>YLSIAFPENTKLDWKPVTKNTRYCPMGGEWFLEPGLQEESFLSSTPIGATPSKSDGFLCHAAKWVTTCDFRWYGPKYITHSIHNIKPTRSDCDTALASYKSGTLVSLGFPPESCGYASVTDSEFLVIMITPHHVGVDDYRGHWVDPLFVGGECDQSYCDTIHNSSVWIPADQTKKNICGQSFTPLTVTVAYDKTKEIAAGGIVFKSKYHSHMEGARTCRLSYCGRNGIKFPNGEWVSLDVKTRIQEKHLLPLFKECPAGTEVRSTLQSDGAQVLTSEIQRILDYSLCQNTWDKVERKEPLSPLDLSYLASKSPGKGLAYTVINGTLSFAHTRYVRMWIDGPVLKEPKGKRESPSGISSDIWTQWFKYGDMEIGPNGLLKTAGGYKFPWHLIGMGIVDNELHELSEANPLDHPQLPHAQS[3x]

Chandipura virus (CHAV, belonging to vesiculovirus genus), is an emerging pathogen associated with deadly encephalitis, principally among children, in India. CHAV single envelope glycoprotein G is involved in two successive steps of virus entry: receptor recognition that allows endocytosis of the virion and fusion of viral and cellular membranes that allows release of the viral nucleocapsid into the cytoplasm for the subsequent steps of infection. As for other rhabdovirus, fusion is triggered at low pH and catalyzed by a conformational change of G from its pre-fusion toward its post-fusion conformation. G ectodomain folds into three distinct structural domains.

In this work, we have characterized the fusion and biochemical properties of CHAV-G and compared them to those of VSV-G. We also determined the structure of a soluble form of CHAV-G ectodomain (CHAV-Gth, generated by thermolysin limited-proteolysis of recombinant VSV particles in which the G gene was replaced by that of CHAV) in the POST conformation at 3.6 Å resolution. In these experiments, we could obtain CHAV-Gth crystals at pH 4.6 and determine the structure of the protein at 3.6 Å resolution by molecular replacement. The single trimer in the asymmetric unit has the three protomers in a classic post-fusion conformation. The three chains were built from residues 1 to 415, 1 to 416 and 1 to 413, for chains A, B and C, respectively; with internal breaks in segments 26–33 and 27–33 of chain A and C. Those breaks reflect the intrinsic flexibility of segment R1. The overall structure of CHAV-Gth is very similar to that of VSVIND-Gth in its post-fusion form. The PHDs are more divergent than FDs and CDs. Only 79 residues of the PHD (called PHD core) out of 90 in CHAV-G are in structurally equivalent positions with VSV-G. The largest differences are confined to helices D and E which are missing in CHAV-G (see the orange arrow on Fig. 3B). A comparison of the sequence of both proteins at these positions reveals that CHAV-G bears an insertion of 4 aa residues at the level of helix E resulting instead in the formation of a small two stranded β-sheet. For CHAV-G, the amino-terminal part of R2 adopts a β-strand conformation, which is followed by a small loop and a small helix; CHAV-G R3 has a structure which is similar to VSV-G R2, a long loop ending in a β-strand.> MESKVVVPAQGKKITLQNGKLNVPENPIIPYIEGDGIGVDVTPAMLKVVDAAVEKAYKGERKISWMEIYTGEKSTQVYGQDVWLPAETLDLIREYRVAIKGPLTTPVGGGIRDLNVALRQELDLYICLRPVRYYQGTPSPVKHPELTDMVIFRENSEDIYAGIEWKADSADAEKVIKFLREEM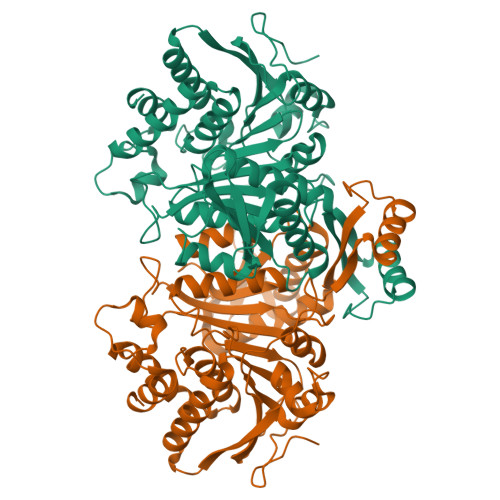GVKKIRFPEHCGIGIKPCSEEGTKRLVRAAIEYAIANDRDSVTLVHKGNIMKFTEGAFKDWGYQLAREEFGGELIDGGPWLKVKNPNTGKEIVIKDVIADAFLQQILLRPAEYDVIACMNLNGDYISDALAAQVGGIGIAPGANIGDECALFEATHGTAPKYAGQDKVNPGSIILSAEMMLRHMGWTEAADLIVKGMEGAINAKTVTYDFERLMDGAKLLKCSEFGDAIIENM>[4x]KDTIALVVSTLNNPFFVSLKDGAQKEADKLGYNLVVLDSQNNPAKELANVQDLTVRGTKILLINPTDSDAVGNAVKMANQANIPVITLDRQATKGEVVSHIASDNVLGGKIAGDYIAKKAGEGAKVIELQGIAGTSAARERGEGFQQAVAAHKFNVLASQPADFDRIKGL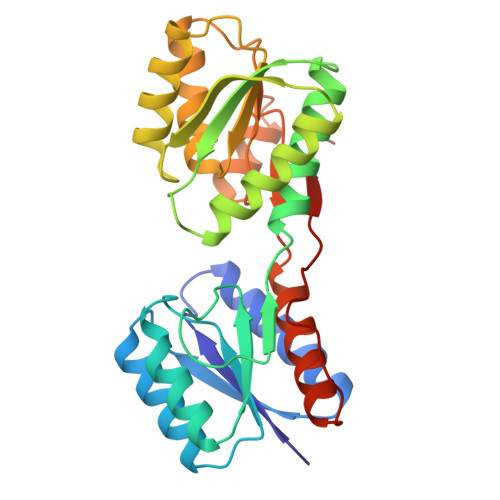NVMQNLLTAHPDVQAVFAQNDEMALGALRALQTAGKSDVMVVGFDGTPDGEKAVNDGKLAATIAQLPDQIGAKGVETADKVLKGEKVQAKYPVDLKLVVKQ> NAVVQLTELGNGVVQITMKDESSRNGFSPSIVEGLRHCFSVVAQNQQYKVVILTGYGNYFSSGASKEYLIRKTRGEVEVLDLSGLILDCEIPIIAAMQGHSFGGGLLLGLYADFVVFSQESVYATNFMKYGFTPVGATSLILREKLGSELAQEMIYTGENYRGKELAERGIPFPVVSRQDVLNYAQQLGQKIAKSPRLSLVALKQHLSADIKAKFPEAIKK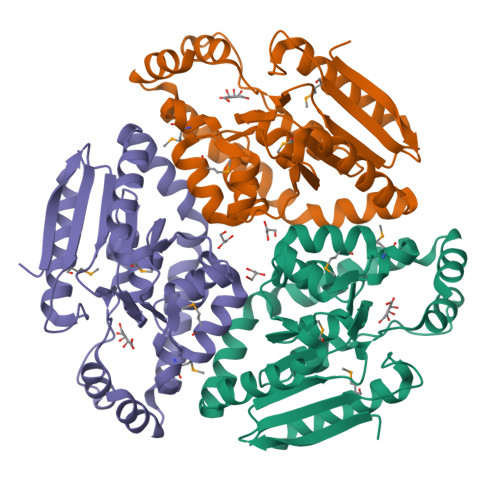ELEIHQVTFNQPEIASRIQQEF> VRERGPQRVAAHITGTRGRSNTLSSPNSKNEKALGRKINSWESSRSGHSFLSNLHLRNGELVIHEKGFYYIYSQTYFRFQEEIKENTKNDKQMVQYIYKYTSYPDPILLMKSARNSCWSKDAEYGLYSIYQ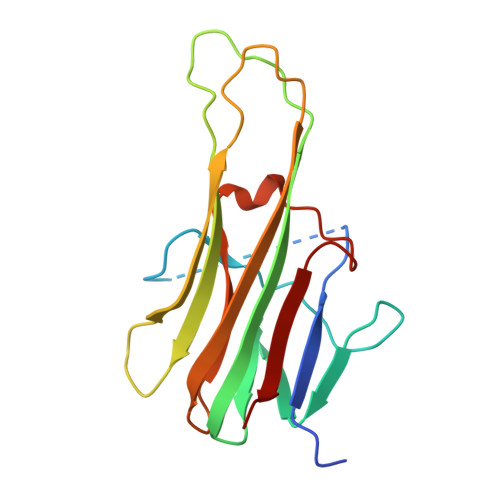GGIFELKENDRIFVSVTNEHLIDMDHEASFFGAFLVG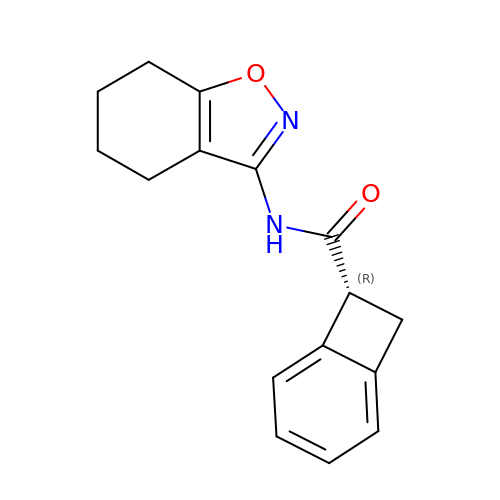(7~{R})-~{N}-(4,5,6,7-tetrahydro-1,2-benzoxazol-3-yl)bicyclo[4.2.0]octa-1,3,5-triene-7-carboxamide | C16 H16 N2 O2 | TVCMRADHQQGKOS-CYBMUJFWSA-N Members of the MenAT family of TA systems in M. tuberculosis encode a toxin with a conserved nucleotidyltransferase (NTase)-like protein domain (DUF1814) and a cognate antitoxin, which can belong to different protein families. We show that MenAT1 can function as a bona fide TA system in vivo in its native host M. tuberculosis. Furthermore, the toxin MenT1 acts as a tRNA NTase in vitro, which transfers CMPs to the 3ʹ end of tRNA acceptor stems without preference for specific tRNAs. MenT1 biochemical activity was fully inhibited by purified MenA1.

We subsequently determined the X-ray crystallographic structure of the MenAT1 complex, to a resolution of 1.44 Å. The MenAT1 crystal structure features two MenT1 protomers (MenT1α and MenT1β) bound to a MenA1 antitoxin monomer to form a MenT1α:MenA1:MenT1β complex. The MenA1 antitoxin protein consists of a long central helix (α1) linked by a flexible loop to a shorter C-terminal helix (α2). The α2 helix folds back, partially towards the α1 helix, yet angled outwards, forming an asymmetrical, twisted “V” shape. Within the complex structure, the resolved MenA1 antitoxin binds asymmetrically, running in opposing directions across the same face of each MenT1 protomer. This brings the electropositive cavities of each MenT1 protomer into juxtaposition, suggesting that MenA1 prevents MenT1 toxicity by blocking the active site. MenA1 residues L14 and V19 bind into pockets lined with L8, L120 and L123 from MenT1α and MenT1β, respectively. A close-up view of the interaction interface reveals that MenT1α F38 is pulled out by the asymmetry of MenA1 binding, allowing formation of a hydrophobic network comprising MenT1α F38, MenT1β F28 and MenT1β F38 stacked underneath MenA1. PDBsum calculated a buried surface area of 895 Å2 between MenA1 and MenT1β, and identified a salt bridge formed between MenA1 R27 and MenT1β E35, supported by hydrogen bonding with MenA1 W47. As such, MenAT1 appears to form a novel complex that is suggested to both sequester and block MenT1 toxins using asymmetric antitoxin binding.

>NAVESTLRRVAKDLTGLRQRWALVGGFAVSARSEPRFTRDVDIVVAVANDDAAESLVRQLLTQQYHLLASVEQDAARRLAAVRLGATADTAANVVVDLLFASCGIEPEIAEAAEEIEILPDLVAPVATTAHLIAMKLLARDDDRRPQDRSDLRALVDAASPQDIQDARKAIELITLRGFHRDRDLAAEWTRLAAKW[2x];> AVSVAAQKLRLALDMYEVGEQMQRMRLGRERPNADVVEIEAAIDAWRMTRPGAEEGDSAGPTSTRFT>GSHMNNEGTKELKLKKLSDNVYQHISYKRVEPWGLIGASGLVVINGTEAHMIDTPWTTQGTKQLIEWIEAKGLTIKSAVVTHFHEDASGDIPLLNDLKIKTYATSLTNKLLKLNQKEVSSDEISSNTFE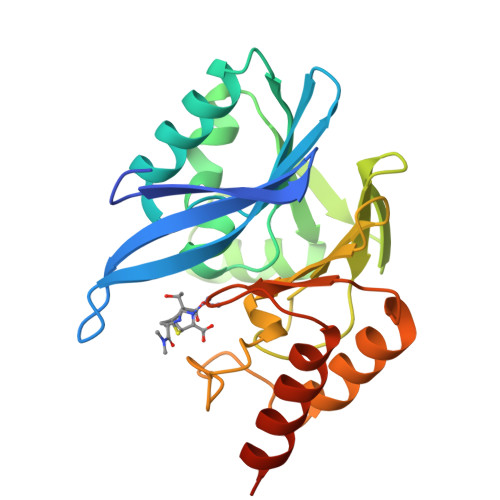FIDGVASVFYPGAGHTEDNIVVWLPNEKILFGGCFVKSLKNKNLGYTGDANISEWPNSMQKVINRYPDAKLVVPGHGEVGDVSLLKHTQALALSAAASNKKINKD[4x]> GAELPAPLRRTGVGEWLATTCQGCTSWCAKQIYVMDGRALKVRGNPNSGVHGMSSCPRQHLSLQQVYDPDRLRTPMMRTNPKKGRDQDPKFVPISWDKALDMLADKIIALRVANEPHKYALLRGRYSHINDLLYKKMTNLIGSPNNISHSSVCAEAHKMGPYYLDGNWGYNQYDVKNAKFILSFGADPIASNRQVSFYSQTWGDSLDHAKVVVVDPRLSASAAKAHKWIPIEPGQDSVLALAIAHVALVEGVWHKPFVGDFIEGKNLFKAGKTVSVESFKETHTYGLVEWWNQALKDYTPEWASKITGIDPKTIIAIAKDMGAAAPAVQVWTSRGAVMQARGTYTSISCHALNGLFGGIDSKGGLFPGNKTPLLKEYPEAKAYMDEIAAKGVKKEKIDQRGRLEFPALAKGKSGGGVITANAANGIR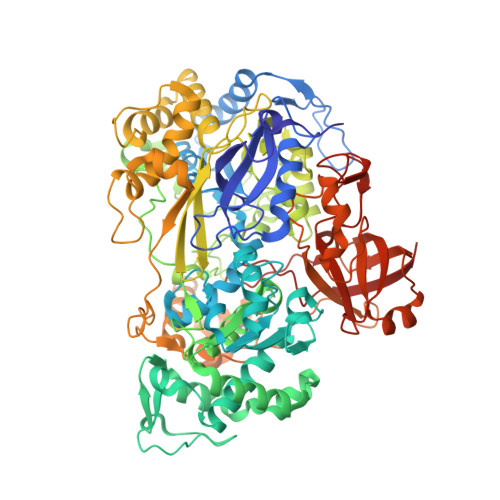NQDPYEIKVMLAYFNNFNFSNPEGQRWDEALSKVDFMAHITTNVSEFSWFADVLLPSSHHMFEKWGVLDSIGNGVAQISIQQPSIKRLWDTRIDESEIPYMLAKKLADKGFDAPWRYINEQIVDPETGKPAADEAEFAKLMVRYLTAPLWKEDASKYGDKLSSWDEFVQKGVWNSSPYKLEARWGKFKTETTKFEFYSKTLEKALQSHADKHKVSIDEVMKACDYQARGHLAFIPHYEEPYRFGDESEFPLLLVDQKSRLNKEGRTANSPWYYEFKDVDPGDVANEDVAKFNPIDGKKFGLKDGDEIRITSPVGMLTCKAKLWEGVRPGTVAKCFGQGHWAYGRYASAKFGVTPRGGSNNDLIADRYDRLSGASAFYGHIRVRVEKV2-[4-[4-[[2-[(2-methylpropan-2-yl)oxycarbonyl]-3-oxidanyl-4-(trifluoromethyl)phenyl]methoxy]phenyl]phenyl]ethanoic 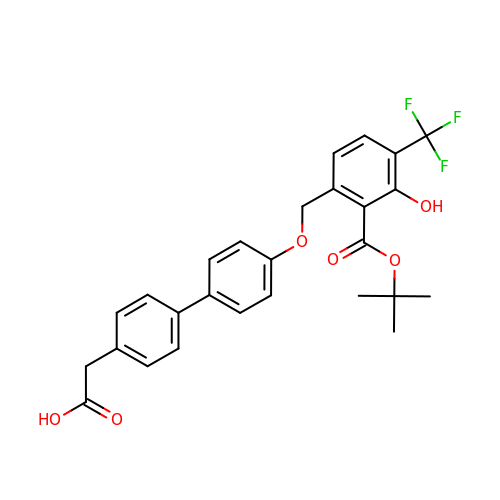acid | C27 H25 F3 O6 | XWHRMVBUKJEZFY-UHFFFAOYSA-N> EQPEPIKVYGQVSLNDSHNQMVVHWAGEKSNVIVALARDSLALARPKSSDVYVSYDYGKSFKKISDKLNFGLGNRSEAVIAQFYHSPADNKRYIFADAYAQYLWITFDFCNTLQGFSIPFRAADLLLHSKASNLLLGFDRSHPNKQLWKSDDFGQTWIMIQEHVKSFSWGIDPYDKPNTIYIERHEPSGYSTVFRSTDFFQSRENQEVILEEVRDFQLRDKYMFATKVVHLLGSEQQSSVQLWVSFGRKPMRAAQFVTRHPINEYYIADASEDQVFVCVSHSNNRTNLYISEAEGLKFSLSLENVLYYSPGGAGSDTLVRYFANEPFADFHRVEGLQGVYIATLINGSMNEENMRSVITFDKGGTWEFLQAPAFTGYGEKINCELSQGCSLHLAQRLSQLLNLQLRRMPILSKESAPGLIIATGSVGKNLASKTNVYISSSAGARWREALPGPHYYTWGDHGGIITAIAQGMETNELKYSTNEGETWKTFIFS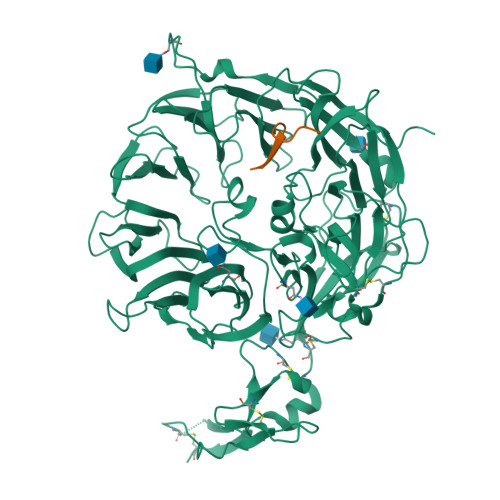EKPVFVYGLLTEPGEKSTVFTIFGSNKENVHSWLILQVNATDALGVPCTENDYKLWSPSDERGNECLLGHKTVFKRRTPHATCFNGEDFDRPVVVSNCSCTREDYECDFGFKMSEDLSLEVCVPDPEFSGKSYSPPVPCPVGSTYRRTRGYRKISGDTCSGGDVEARLEGELVPCPSRLENLYFQ;> LPQDRGFLVVQGDPR> GPGMTIKGSGSAAFEGTRLCPRVIKPDGPATILAIGTSNPTNIFEQSTYPDFFFDVTNCNDKTELKKKFQRICDKSGIKKRHFHLTDEILRKNPSICKFKEASLDPRQDIAVLEVPKLAKEAAISAIKQWGQPKSKITHLVFATTSGVDMPGADFQLAKLLGLRPTVKRVMLYQQGCYAGATVLRVAKDLAENNKGARVLVACSEVTAVTFRAPSETHLDGLVGSALFGDGAAALIVGSDPVPQEEKPLFEIHWAGEAVLPDSDGAIN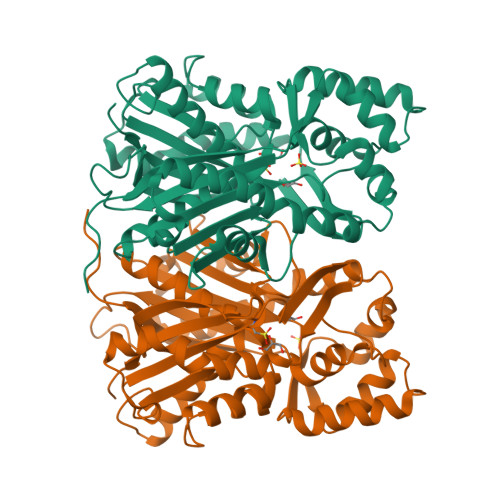GHLREAGLIFHLLKDVPGLISKNIDKVLAEPLEYVHFPSYNDMFWAVHPGGPAILDQIEAKLGLSTDKMQASRDVLASYGNMSSASVLFVLDQIRKNSEELHLPTTGEGFEWGFVIGFGPGLTVETLLLRSINI> GSHMNGRIYAVGGYDGSPDGHTHLNSVEAYDPETDTWSPVAPMNTRRSGVGVAVLDGHIYAVGGSHGSPDGSIHHNSVERYEPERDEWHLVAPMLTRRIGVGVAVLNGRIYAVGGYDGSPDGHTHLNSVEAYDPETDTWSPVAPMNTRRSGVGVAVLDGHIYAVGGSHGSPDGSIHHNSVERYEPERDEWHLVAPMLTRRIGVGVAVLNGRIYAVGGYDGSPDGHTHLNSVEAYDPETDTWSPVAPMNTRRSGVGVAVLDGHIYAVGGSHGSPDGSIHHNSVERYEPERDEWHLVAPMLTRR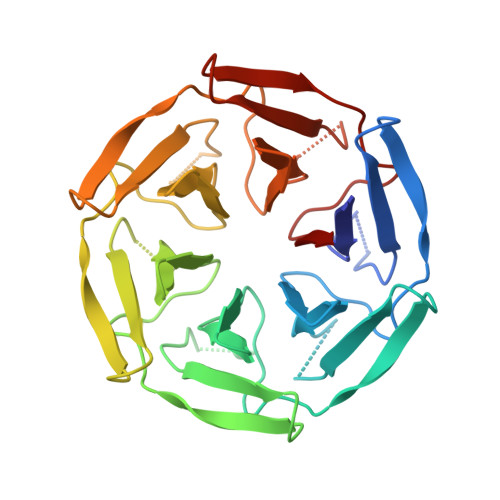IGVGVAVL>MTERIRNVALRSKVCPAETASELIKHGDVVGTSGFTGAGYPKEVPKALAQRMEAAHDRGEKYQISLITGASTGPQLDGELAKANGVYFRSPFNTDATMRNRINAGETEYFDNHLGQVAGRAVQGNYGKFNIALVEATAITEDGGIVPTSSVGNSQTFLNLAEKVIIEVNEWQNPMLEGIHDIWDGNVSGVPTRDIVPIVRADQRVGGPVLRVNPDKIAAIVRTNDRDRNAPFAAPDETAKAIAGYLLDFFGHEVKQNRLPPSLLPLQSGVGNVANAVLEGLKEGPFENLVGYSEVIQDGMLAMLDSGRMRIASASSFSLSPEAAEEINNRMDFFRSKIILRQQDVSNSPGIIRRLGCIAMNGMIEADIYGNVNSTRVMGSKMMNGIGGSGDFARSSYLSIFLSPSTAKGGKISAIVPMAAHVDHIMQDAQIFVTEQGLADLRGLSPVQRAREIISKCAHPDYRPMLQDYF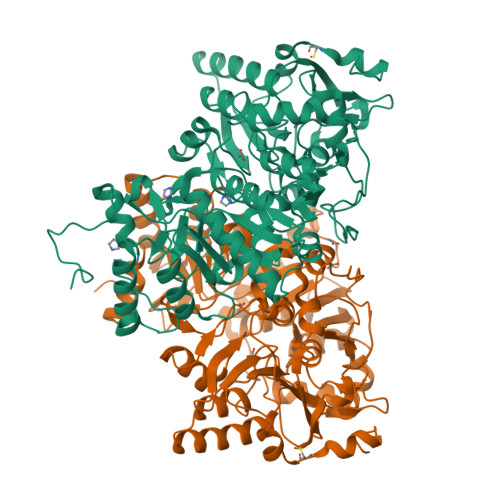DRALKNSFGKHTPHLLTEALSWHQRFIDTGTMLPSSLEHHHHHH[2x]Self-labeling protein tags such as HaloTag are powerful tools that can label fusion proteins with synthetic fluorophores for use in fluorescence microscopy. Here we introduce HaloTag variants with either increased or decreased brightness and fluorescence lifetime compared with HaloTag7 when labeled with rhodamines. To engineer the binding site, ten amino acids on helices 6–8 in close proximity to TMR were chosen for randomization by site-saturation mutagenesis. The changes in spectroscopic properties result from single or double point mutations in the direct vicinity of the bound fluorophore.

The brightest variant, the double mutant HaloTag9 (HaloTag7-Q165H-P174R, ΔI = 19.9 ± 0.5%), as well as the dimmer variants HaloTag10 (HaloTag7-Q165W, ΔI = −52.9 ± 1.2%) and HaloTag11 (HaloTag7-M175W, ΔI = −44.8 ± 0.8%) were chosen for characterization with a panel of 46 different fluorophores and analysis of their photophysical properties. HaloTag10 and HaloTag11 decreased the fluorescence intensity of almost all tested fluorophores compared with HaloTag7. The decreases were more pronounced for HaloTag10 than for HaloTag11 but in both cases caused by changes in quantum yield. For HaloTag10 and HaloTag11, the proximity of TMR to the introduced tryptophans suggests that photoinduced electron transfer (PET) quenching of the fluorophore is responsible for the decreased quantum yields. The decreased quantum yields and fluorescence lifetimes of HaloTag10 and HaloTag11 presumably result from PET quenching through the newly introduced tryptophans. Hence, HaloTag9 showed the longest and HaloTag10 the shortest fluorescence lifetime. HaloTag10 and HaloTag11 decreased the brightness of all fluorophores relative to HaloTag7, HaloTag10 having the biggest effect. Photostability measurements showed that the higher the fluorescence lifetime, the more photobleaching occurred, making HaloTag9 the least and HaloTag10 and HaloTag11 the most photostable tags.

>GIGTGFPFDPHYVEVLGERMHYVDVGPRDGTPVLFLHGNPTSSYVWRNIIPHVAPTHRCIAPDLIGMGKSDKPDLGYFFDDHVRFMDAFIEALGLEEVVLVIHDWGSALGFHWAKRNPERVKGIAFMEFIRPIPTWDEWPEFARETFQAFRTTDVGRKLIIDWNVFIEGTLPMGVVRPLTEVEMDHYREPFLNPVDREPLWRFPNELPIAGEPANIVALVEEYMDWLHQSPVPKLLFWGTPGVLIPPAEAARLAKSLPNCKAVDIGPGLNLLQEDNPDLIGSEIARWLSTLEI[6x]>[3x]PSNMKQFCKISVWLQQHDPDLLEIINNLCMLGNLSAAKYKHGVTFIYPKQAKIRDEIKKHAYSNDPSQAIKTLESLILPFYIPTPAEFT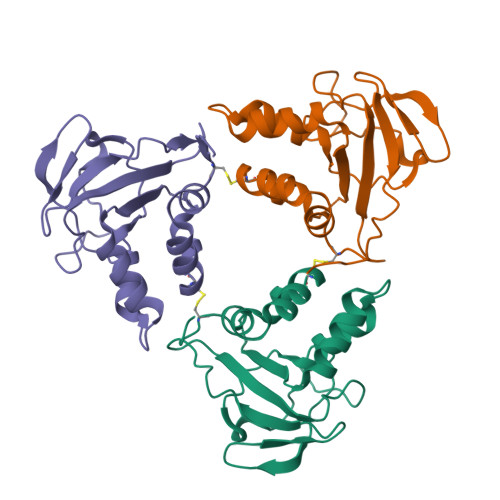GEIGSYTGVKLEVEKTEANKVILKNGEAVLVPAADFKPFPDRRLAVWIMESGSMPLEGPPYKR> MRGLAVLVLLVFAVQVAAAEDFRPVVFVHGLAGSAGQFESQGMRFAANGYPAEYVKTFEYDTISWALVVETDMLFSGLGSEFGLNISQIIDPETLDKILSKSRERLIDETFSRLDRVIDEALAESGADKVDLVGHSMGTFFLVRYVNSSPERAAKVAHLILLDGVWGVDAPEGIPTLAVFGNPKALPALGLPEEKVVY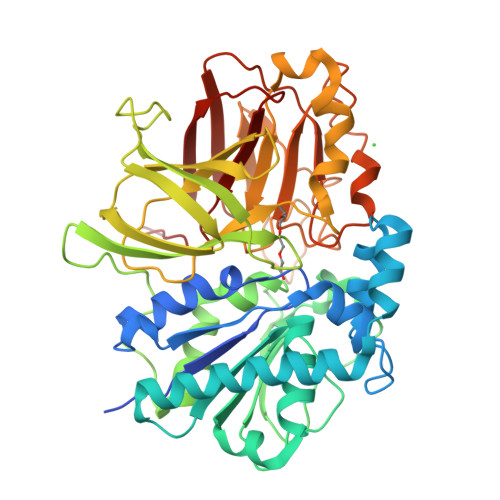NATNVYFNNMTHVQLCTSPETFAVMFEFINGYKPATTDIVPQDGDYVKVKGKFLAFATNGDVSGWLSIYPIDENGKRLTRLPVKFMRVKGDFEVRLRKGQLYEFQFRKDFSPIIYHYYRAPFVRDDLWARFLVSKPPLDVELLILPERLSPAAKETSGLLLIRYKEMIGEYDEEIGGVDEVYVNGVNVCTERICPIERAVNGLWVFDRGADGKSDLDREVVRYSIMPFMSAADLVVPAEGTISIAVKSRTGGEESFTIPAWSADRHSIIVQFSDYIVDKLA> VTDLAGTTRLLRAQGVTAPAGFRAAGVAAGIKASGALDLALVFNEGPDYAAAGVFTRNQVKAAPVLWTQQVLTT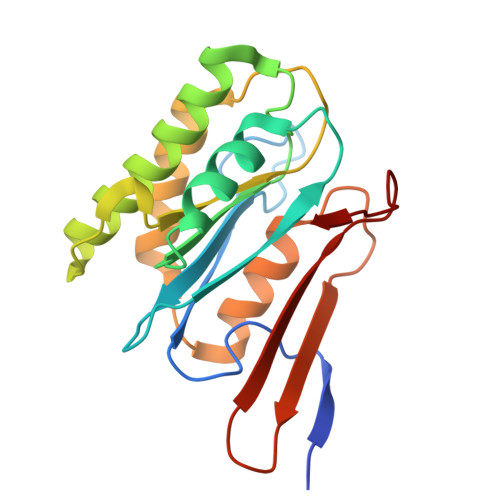GRLRAVILNSGGANACTGPAGFADTHATAEAVAAALSDWGTETGAIEVAVCSTGLIGDRLPMDKLLAGVAHVVHEMHGGLVGGDEAAHAIMTTDNVPKQVALHHHDNWTVGGMAKGAGMLAPSLA>CPQNCHCHSDLQHVICDKVGLQKIPKVSEKTKLLNLQRNNFPVLAANSFRAMPNLVSLHLQHCQIREVAAGAFRGLKQLIYLYLSHNDIRVLRAGAFDDLTELTYLYLDHNKVTELPRGLLSPLVNLFILQLNNNKIRELRAGAFQGAKDLRWLYLSENALSSLQPGALDDVENLAKFHVDRNQLSSYPSAALSKLRVVEELKLSHNPLKSIPDNAFQSFGRYLETLWLDNTNLEKFSDGAFLGVTTLKHVHLENNRLNQLPSNFPFDSLETLALTNNPWKCTCQLRGLRRWLEAKASRPDATCASPAKFKGQHIRDTDAFRSCKFPTKRSKKAGRH[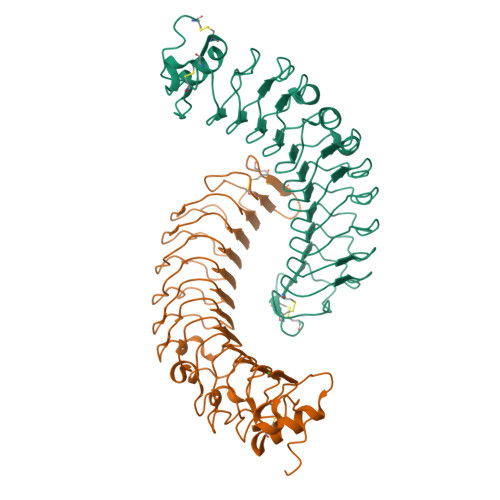4x]CISs are macromolecular injection devices with an overall structure that is homologous to the contractile tails of bacteriophages. Their conserved modules include an inner tube, a contractile sheath and a baseplate complex. For firing of the extended apparatus, the baseplate undergoes a conformational change and triggers sheath contraction, which in turn causes the inner tube to be expelled and injected into a target. Here we performed structural and mechanistic studies on a clade Ib CIS gene cluster in the marine bacterium Algoriphagus machipongonensis PR1.

Six protofilaments of sheath proteins adopt a right-handed helical array with a length of 92.4 nm and an outer diameter of 24.6 nm. Unlike the multiple sheath proteins present in PVC/AFP, the AlgoCIS sheath is composed of only one protein, Alg2, which folds into four domains. The conserved domains I and II contribute to the sheath wall, with additional domains III and IV extending outwards. The sheath subunits are interwoven with each other via a conserved ‘handshake’ and iteratively assemble into the full sheath, where the attachment helix in domain I mediates the interactions with the inner tube. Interestingly, depending on its location in the different sheath layers, Alg2 exhibits pronounced structural variations. The hinge angles of domain IV were also observed to be different when comparing the different Alg2 layers. A lowpass-filtered map indicates that there are two potential conformations of domain IV in the central sheath layers. The inner tube subunits possess the conserved β-barrel structures and the N terminus of Alg1 is shorter than that of Pvc1 and Afp1.

>[18x]MATYKTPGVYIEEITKFPPSVAQVETAIPAFIGYTQFARTKPSVDSDDLILKPKRISSLLDFTTYYGGAQNEQGITVKLTDTLIEGAENRTINVPEPTFKSPYLMFYSLQMYFANGGGPCYIVSTGVYDDWSDSETPPTINFSDLESGLAVIRKEDEPTLLLFPDATNLPTDDEFYSLYNSALMQCNDLQDRFTILDTYSDQTYNDGVEDLDPIPALRNGINLTKDYLKYGAAYYPFVQTILNYQYSADEIVIQHLSYNPNAIATALDNLNAVNGPTFIDAILDDLRDLSLPDISGEISDAVGFMYDDVDGFDIDGTFTTNSVKVANFASLVESVLSTLNELIDAKEEINKDVNSAIASSEEDNAIKTAISDALDVFNEDFEGADKIESVAKNLSDLLIKIKQADTNTKVENVLSINALNFSAEFEKLLTYDVNTGLTASVTLDLFANIGTRLDDIIAAVSAAEPIDVNNGKLNGRLLSDIEPLDNATYNTILLEINSHKVTLPPSSSMAGAYARVDNDRGVWKSPANIGLNYVSKPSVTVSHEEQESMNVHGTGKSVNAIRSFVGKGTLVWGARTLAGNDNEWRYISVRRFFNMAEESIKKATEQFVFEPNDGNTWVRVRAMIENFLILQWRAGALAGAKPEHAFYVKVGLGQTMTAQDILEGNMNVEIGLAVVRPAEFIILKFSHKMQES;>MSYPLSKFHFSVEWGGTKIGFTEVSGLDLETEIIEYRHGASPEYSKIKMPGMQKFSNITLKRGTFKSDNEYFQWYNTINLNKVERRDLTISLLNEEHEPVVTWKVKNAWPLKVQSTDLKGDGNEVAIESMELAHEGLVIQNE[18x]> MALYPIKSLGAVGVIADQAPTDLAPNAFTNAINARFVEQRVFKTGGNAPLSYVDEDKDLTPLSFVSMPFDYYSAGNSFLVVGTNKKLYKLTDESLTDISRKVATVTKKASASIKIYPVVSQIVPKESTISMNFNQTKNLEVSLLPADANNTNLIWEVSNSSYGSITVDPSDSKLATLTSFEKEGNLVVTISTANESVVAQIAVNIIDGDSGIFLSQDTVTIRKGGTTTLTAVTGKTPVTWSSNNASIVSVTPNANSLTAVITANGEGNVTITADNGTKTASCEIVSIPQIDSISLSQSDVTVSRGSQYILTATLSPANAPNQNITWTSSNPNIATVSGTSTQGTINALLAGFTEITATTEEGNRVAVCTVRVDLAGRTMRTSAMAFAAPVSESVETQEEEVVTPPESEETVYFAEPTSGIDTSGMYEGNNFYDYSNVNDIEGFARASLLATPLSSVTLDIVSASLDVGEEIVITATASPEGEYSYQWSVDKTGYVSTTSVTGKSIKLVALRKGEINVTCTVSQMTQKDYDAFDDYPWYHAVISNCAVATTHYETPQVKEFESEYFVDLPGWGEQTVVDNDGNPSVKKFNWKCERVRSFNNRLFALNMREANASGVTTNYPLRLRWSNFANENKAPTLWDDFAYDRVVSSDLASNIVGQTQALENGYAGYIDLADSNGSLIDILPLKDYLFVYTEFETYIGSPTNNTYQPLMFKKLFNDSGILAPECVVEVEGSHFVVTQNDVILHNGATKKSIASNRVKNMLINEVCLVNPLATRVHLHQDKKEVWVLYVGPGEPKESFACTKAAVWNYEFDTWSFRTIPYAQCIGLVDPPVLERGPIWSDFQEITWDDPSIKELVWRKDATNFRQRVTIVGSFLKGFYQVDVGALDYFYDRLNDVVIEKPLEMRLERTGI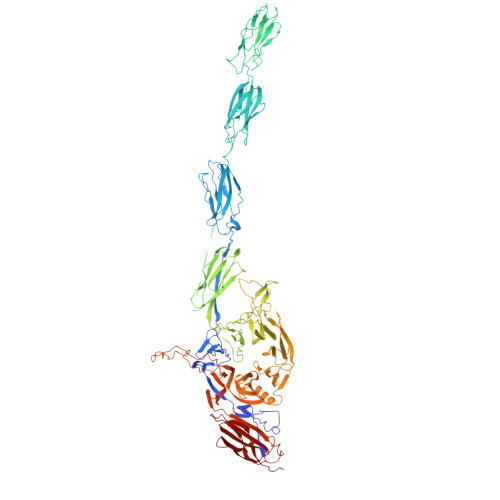DFDNVTNEWNQKHINRFRPQTTGSGTYIFEAGGSQFSNEYGHPHTSKTYTIGVDRHVSVRLNHPYLFYNVIDNDVNSNAAINGLTIEFAVGGRR> GPLGSPDYGN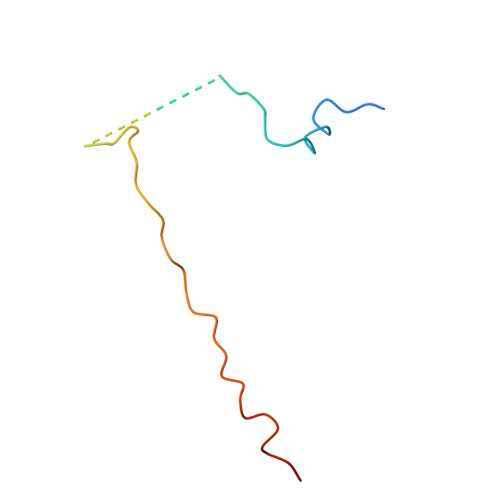SALLSLPGYRPTTRSSARRSQAGVSSGAPPGRNSFYMGTCQDEPEQLDDWNRIAELQQRNR Mutations in the human PURA gene cause the neurodevelopmental PURA syndrome. Based on the crystal structures of PURA from Drosophila melanogaster (dmPURA), three conserved sequence regions termed PUR repeats I, II, and III were identified to fold into globular domains. Whereas PUR repeat I and II assemble into an N-terminal PUR domain via intramolecular interactions, two C-terminal PUR repeats III from different molecules interact with each other and thus mediate dimerization of PURA. All these PUR domains belong to the class of the PC4-like protein family, which mainly bind single-stranded nucleic acids and can unwind double-stranded DNA and RNA.

CD spectra had already suggested that this mutation has no dramatic effect on the overall domain folding. To assess if this variant has a rather local effect on the structural integrity of PURA that may not be detectable by CD spectroscopy, we solved the crystal structure of hsPURA I–II R140P at 2.15 Å resolution. The crystals of R140P variant protein exhibited the same space group, unit cell parameters, and crystal packing as the wild-type protein. The R140P variant is located at the end of the flexible linker between PUR repeats I and II connecting helix α1 to the strand β5. Because of its position in a flexible region, the mutated residue is partially visible only in one out of four PURA chains in the asymmetric unit. The overlap of the R140P-variant structure with the PURA I–II WT fragment confirmed our previous observation about the unusually high flexibility of the strands β4 and β8 forming the β-ridge. Since no major structural differences were visible between hsPURA I–II WT and R140P variant (average r.m.s.d. of 0.89 Å for 133 Cα atoms aligned), we concluded that this genetic variation is unlikely to impair the structural integrity of hsPURA. In contrast, hsPURA I–II R140P did not show impaired RNA binding. In contrast, hsPURA I–II R140P variant showed wild-type-like separation of dsDNA, further supporting our previous interpretation from RNA-binding analyses that the genetic variant R140P is likely functional.

>ETQELASKRVDIQNKRFYLDVKQNAKGRFLKIAEVGAGGNKSRLTLSMSVAVEFRDYLGDFIEHYAQLGPSQPPDLAQAQDEPPRALKSEFLVRENRKYYMDLKENQRGRFLRIRQTVNRGPGLGSTQGQTIALPAQGLIEFRDALAKLIDDYGVE[4x]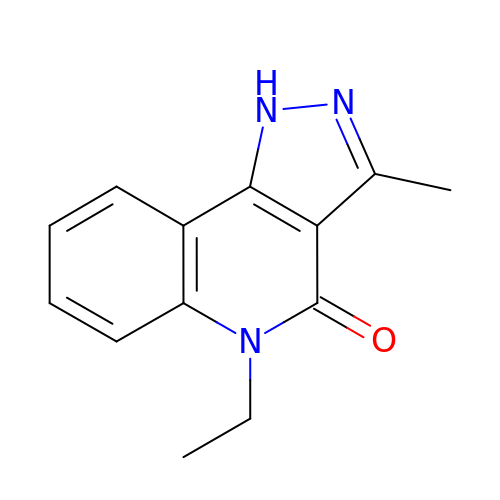5-ETHYL-3-METHYL-1,5-DIHYDRO-4H-PYRAZOLO[4,3-C]QUINOLIN-4-ONE | C13 H13 N3 O | ASEHARDUZDZEKS-UHFFFAOYSA-N>[3x]MKKKGSVVIVGRINLSGDTAYAQQTRGEEGCQETSQTGRDKNQVEGEVQIVSTATQTFLATSINGVL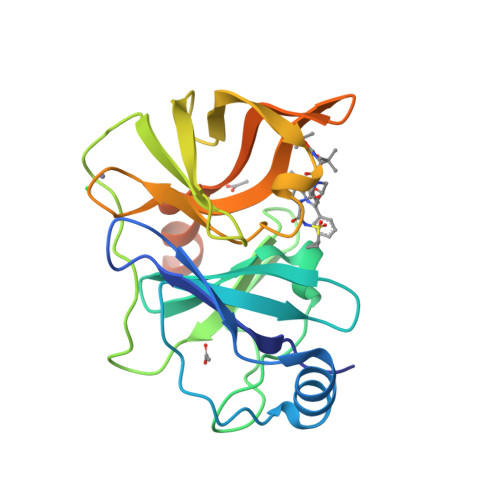WTVYHGAGTRTIASPKGPVTQMYTNVDKDLVGWQAPQGSRSLTPCTCGSSDLYLVTRHADVIPVRRRGDSRGSLLSPRPISYLKGSSGGPLLCPAGHAVGIFRAAVCTRGVAKAVDFIPVESLETTMRSPAIRAPSTSLRPHSSTTTTTTEI>[2x]QQASTLPDLAEQFAPPDVAPPLLIKLVEAIEKKGLECSTLYRTQSSSNPAELRQLLDCDTASLDLEMFDVHVLADAFKRYLLDLPNPVIPVAVSSELISLAPEVQS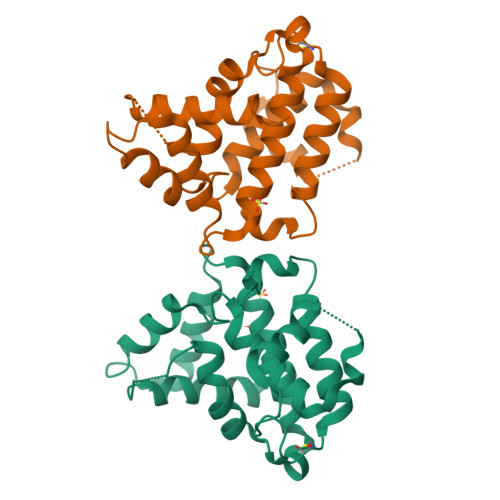SEEYIQLLKKLIRSPSIPHQYWLTLQYLLKHFFKLSQTSSKNLLNATVLSELFSPLLFRFPAASSENTEHLIKIIEILISTEWNERQ N-[6-(4-ethylpiperazin-1-yl)-2-methyl-pyrimidin-4-yl]-5-pyridin-4-yl-1,3-thiazol-2-amine | C19 H23 N7 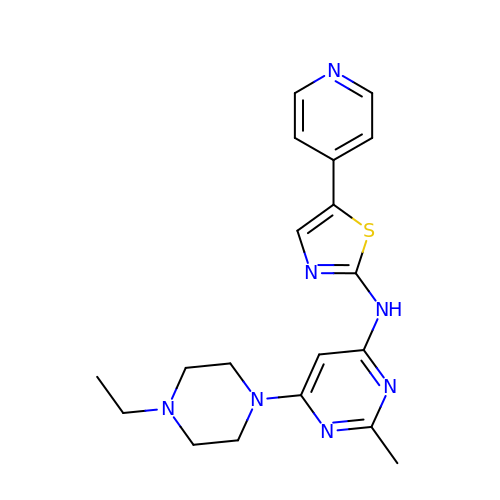S | MBWHJBDHRADERX-UHFFFAOYSA-N> GDNKGITYEELNPERFTLLEKGTPTNILIDENEDQGVMIAATNLSEDFGRVSGTNAPLIFLPDNERLIIVGTLESRYIKELTENRKIKGDELKGKNEKYLMTVVDNPLPGVKEALIIAGSDKRGAIYGIYELSEQIGVSPWYDWADVPVKPQQNLSIERGSYTADEPAVTYRGIFLNDEAPALTSWVENTYGTKYGDHRFYSRVFELILRLRGNFLWPAMWDWSFYGDDPLNSKTADTMGIIMGTSHHEPMARNHQEWARNRDKYGVWDYTSNQEVIDQFFREGIERVKDTDDLITIGMRGGDGATPMGVKEGEDHLFVSDEDNMRLLERIIKNQREIIGDVTGESPEKTPQVWAIYKEVQRYFDLGLRPPEDVIILLSDDNWGNVRRLPTEEERDHPGGWGMYYHFDYVGAPRSSKWLNISPIQNIWEQMQLTYDYGVDELWVANVGDLKPMEYPITLFLDMAWDPTRFNAENLLDHTRSFAAQQFGEDQADEAARIINLYSKYNGRVTPEMLDRNTYNLESGEWKKVSDEYIKLEAEALRQYLTLEPEQRDAYKQLILYPVQAMANLYEMYYSQAMNHKLYRENNPMANYWADRVEETFNRDAELSHDYNKVMANGKWDGMMTQKKIGYRSWNDNFPADTLPQIFRIENPEEATGGYVFTARDGVVVIEAEHYFEAKDAEEAKWTVIPYMGRTLSSIALMPYTKEVEGASLSYRMQIPDEVSEVKVHVVVKSTLPFHDPKGHEYRVGFEGGSKEIVNFNWNLNEEPENIYSVFYPTVASRVVKKDVTLDLHDTDDGFYTLTLEPLDPGIVFQKIVVDFGGYEESRLFMEESPNKRIEES

The xylan-specific α-glucuronidases from glycoside hydrolase family 115 (GH115) specifically catalyse the removal of α-d-glucuronic acid (GlcA) or methylated GlcA (MeGlcA). In this study, we report crystal structures of a bacterial GH115 ortholog (wtsAgu115A) identified in a metagenome from an anaerobic digester fed with wastewater treatment sludge. Furthermore, wtsAgu115A eluted from a gel-filtration column at a volume consistent with a dimer in solution, which suggests that wtsAgu115A is a dimer in its active form similar to other GH115 xylan-specific α-glucuronidases.

Three Ca2+ ions were modelled in wtsAgu115A D303A in the unbound form. However, two of these are found on the surface of the enzyme and are likely to originate from the crystallization conditions, which contained 0.2 M CaCl2. A structural comparison between unbound wtsAgu115A D303A and wtsAgu115A–xylohexaose yields an overall r.m.s.d. of 0.17 Å for Cα atoms, which suggests that the binding of xylohexaose does not impose any major domain conformational changes in wtsAgu115A.N-methyl-N-phenyl[(3aM)-3-(trifluoromethyl)cyclopenta[c]pyrazol-2(1H)-yl]ethanethioamide | C16 H14 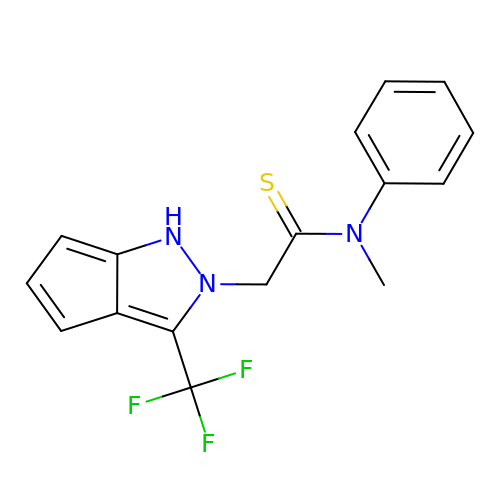F3 N3 S | HKIQFXYWIJQJAT-UHFFFAOYSA-N> GSHMTVREQDRFMPIANVIRIMRRILPAHAKISDDSKETIQECVSEYISFITGEANERCQREQRKTITAEDVLWAMSKLGFDDYIEPLTLYLHRYRE;> MTQFKEIEKTTDFKNHSLPLARIKKIMKADEDVRMISAEAPVVFARACEMFILELTLRSWNHTEENKRRTLQKNDIAAAVTRT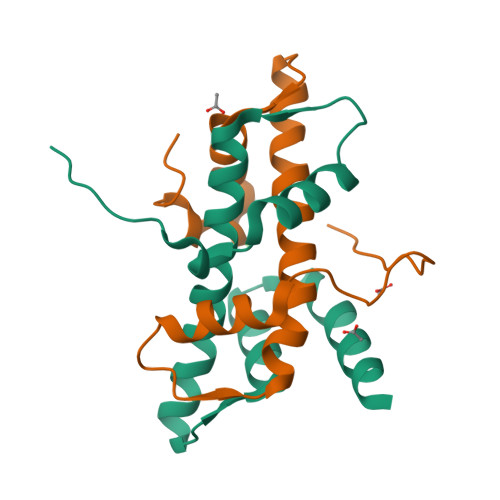DIFDFLVDIVPR> MFRLNSLSALAELAVGSRWYHGGSQPIQIRRRLMMVAFLGASAVTASTGLLWKRAHAESPPCVDNLKSDIGDKGKNKDEGDVCNHEKKTADLAPHPEEKKKKRSGFRDRKVMEYENRIRAYSTPDKIFRYFATLKVISEPGEAEVFMTPEDFVRSITPNEKQPEHLGLDQYIIKRFDGKKISQEREKFADEGSIFY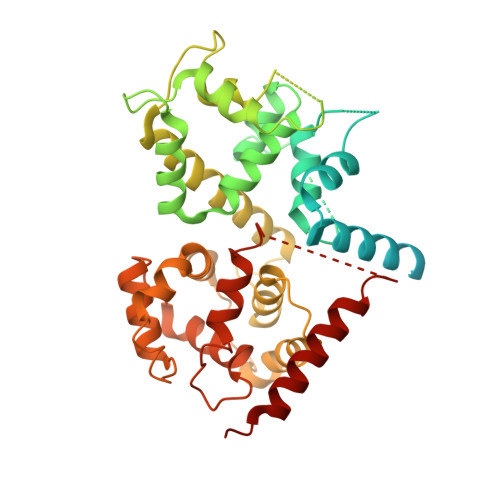TLGECGLISFSDYIFLTTVLSTPQRNFEIAFKMFDLNGDGEVDMEEFEQVQSIIRSQTSMGMRHRDRPTTGNTLKSGLCSALTTYFFGADLKGKLTIKNFLEFQRKLQHDVLKLEFERHDPVDGRITERQFGGMLLAYSGVQSKKLTAMQRQLKKHFKEGKGLTFQEVENFFTFLKNINDVDTALSFYHMAGASLDKVTMQQVARTVAKVELSDHVCDVVFALFDCDGNGELSNKEFVSIMKQRLMRGLEKPKDMGFTRLMQAMWKCAQETAWDFALPKQ>[2x]KREVRLMKNREAARESRRKKKEYVKS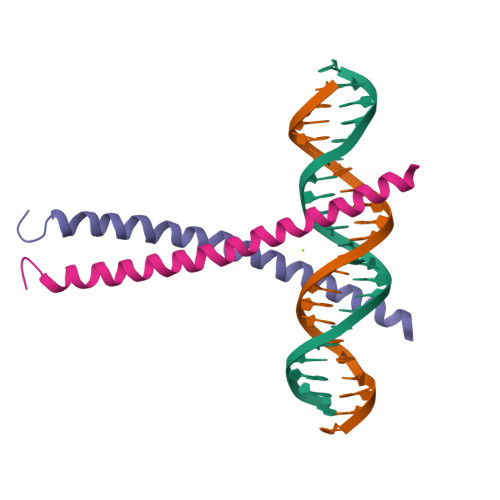LENRVAVLENQNKTLIEELKALKDLYSHK DMHBO+ | C22 H25 N4 O5 | 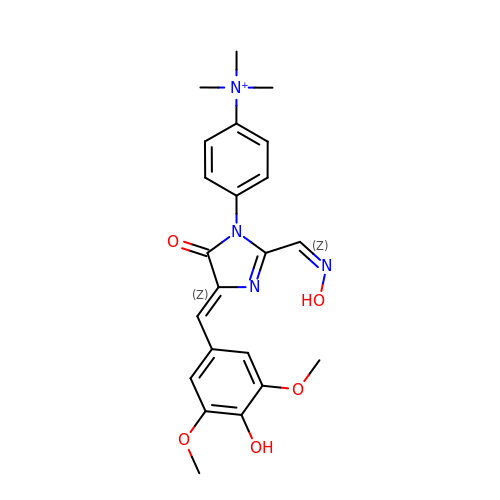GYWNIEJGWAVLAZ-UHFFFAOYSA-O> GSTENDEYKKDSPSAENPAEPVGALLEDFSIEQLPAKTIYALGE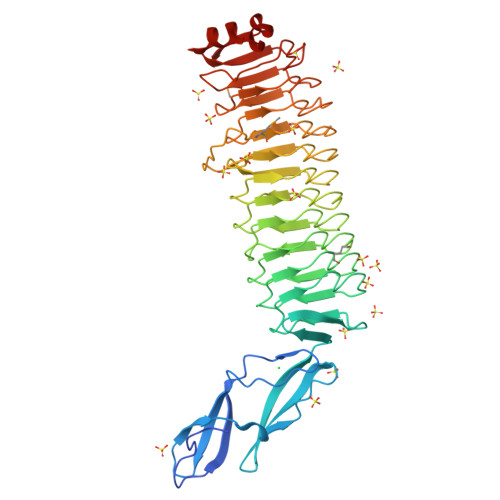NIDLTGLNVTGKYDDGKQRPVKVTPEQISGFSSSAPVDKQEVTITIEGKQKSFSVQISPVRVENGVLTEVLKGHNEIILPNSVKSIPKAAFRGSQINKVVLNEGLQSIGDMAFFNSTVQEVVFPTTLEQLEENIFYYCRNLKKADLSRTKLTKLPASTFVYAGVEEVLLPATLKEIGAQAFLKTSQLKTIEIPENVRTIGLEAFRESGITTVKLPNGVTTIAQRAFYYCPELTEVTTYGTVINENPEAMIHPYCLEGCPKLTRFDISKSIRILGQGLLGGNRKVTQLTIPANVTQINFSAFNNTGIKEVMVEGITPPQVFEKVWYGFPDDITVIRVPAESVEKYKNANGWKDFTNKITAF> MGPKSAPLKEIPDVLVDPRTMKRYMRGRFLGKGGFAKCYEITDMDTKEVFAGKVVPKSMLLKPHQKEKMSTEIAIHKSLDNPHVVGFHGFFEDDDFVYVVLEICRRRSLLELHKRRKAVTE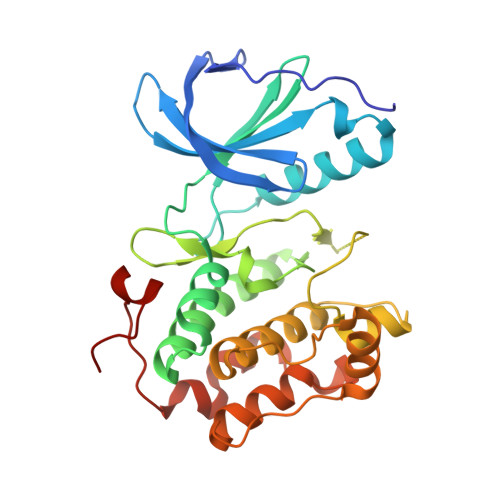PEARYFMRQTIQGVQYLHNNRVIHRNLKLGNLFLNDDMDVKIGDFGLATKIEFDGFRKKTLCGTPNYIAPEVLCKKGHSFEVDIWSLGCILYTLLVGKPPFETSCLKETYIRIKKNEYSVPRHINPVASALIRRMLHADPTLRPSVAELLTDEFFTSGYAPMRLPTSCLTVPPRFS Lipid transfer proteins (LTPs), also called non-specific lipid transfer proteins (nsLTPs), are known for their ability to bind and transport hydrophobic ligands. The biological role of nsLTPs is still not well understood. They transport these lipids between biological membranes primarily for defense, including structural adaptation, antimicrobial activity, and pathogenic resistance. We elucidated the crystal structures of Act c 10.0101 and Pun g 1.0101, nsLTP allergens from gold kiwifruit and pomegranate, respectively. These allergens both belong to the subfamily of 9-kDa LTPs.

Pun g 1.0101 also crystallized in the P21 space group; however, the asymmetric unit contains four protein molecules. The model was refined to 2.4Å resolution. The protein molecules forming the crystal have the sequence that corresponds to Pun g 1.0101, and all four chains include all 93 residues. Similar to Act c 10.0101, the structure of Pun g 1.0101 is stabilized by four disulfide bridges formed by residues Cys4–Cys52, Cys14–Cys29, Cys30–Cys75, and Cys50–Cys89. However, the conformations of the protein molecules present in the asymmetric unit differ, and half of the molecules have a distinct conformation corresponding to residues 77–85. This stretch of the polypeptide chain controls the opening of the ligand binding cavity and corresponds to the Ω loop. Chains A and B adopt one conformation, and chains C and D adopt the second observed conformation. Despite the different conformations, none of the protein chains have a ligand bound; therefore, the crystal structure provides insight into the structure of two Pun g 1.0101 apo forms. In the case of chains A and B, cavities with volumes of approximately 370 and 340 Å3 are observed, and in the case of chains C and D, the cavity volume is ~414 Å3. The difference in likely modes of ligand binding for Act c 10.0101 is not only related to the presence of the conserved aspartic acid residue in kiwifruit protein, but also the absence of a tyrosine residue in the Ω loop. This tyrosine (residue 81) is present in Pun g 1.0101 isoallergens, and it was shown to significantly change conformation after ligand binding.

>AVTCGQVASSLAPCIPYARSAGGAVPPACCSGIKTLDGMARTTPDRQATCKCLKSASTSISGINYGLVASLPAKCGVNIPYKISPSTDCARVK[4x]>MSLASHPPIPILELADHIERLKANDNLKFSQEYESIDPGQQFTWEHSNLEVNKPKNRYANVIAYDHSRVLLSAIEGIPGSDYVNANYIDGYR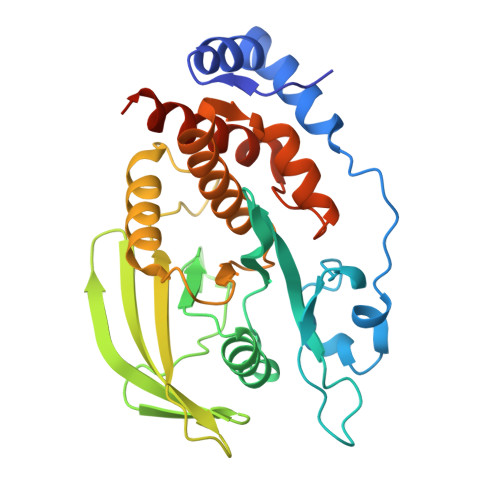KQNAYIATQGSLPETFGDFWRMIWEQRSATVVMMTKLEERSRVKCDQYWPSRGTETHGLVQVTLLDTVELATYCVRTFALYKNGSSEKREVRQFQFTAWPDHGVPEHPTPFLAFLRRVKTCNPPDAGPMVVHCSAGVGRTGCFIVIDAMLERIKHEKTVDIYGHVTLMRAQRNYMVQTEDQYIFIHDALLEAVTCGNTEEGHHHHHH[3x]>[4x]SMMKRLEGKSALITGSARGIGRAFAEAYVREGATVAIAD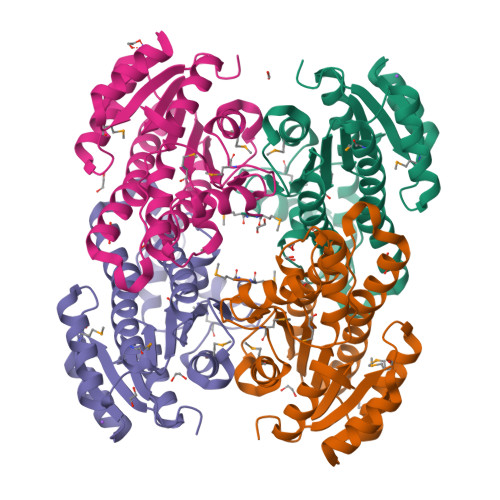IDIERARQAAAEIGPAAYAVQMDVTRQDSIDAAIAATVEHAGGLDILVNNAALFDLAPIVEITRESYEKLFAINVAGTLFTLQAAARQMIAQGRGGKIINMASQAGRRGEALVAIYCATKAAVISLTQSAGLDLIKHRINVNAIAPGVVDGEHWDGVDALFARYENRPRGEKKRLVGEAVPFGRMGTAEDLTGMAIFLASAESDYIVSQTYNVDGGNWMS> MIVFRYLSREVLVTMSAVSAVLLVIIMSGRFIKYLAQAAQGLLDPGSLFLIMAFRIPGFLQLILPLGLFLGILLAYGRLYLESEMTVLSATGMSQKRLLGYTMAPALLVAILVAWLSLFLAPQGINQFALLLNKQDTLTEFDTLVPGRFQAMRDGTRVTYTEELSKDRGELAGIFISQKDLNSSNQERGISILVAEKGTQNIQADGSRYLILHNGYRYDGNPGQANYRAIQYDTYGVMLPKPEASSEVSERDAVPTADLFGSDNPRYQAELQWRLSTPLLVFVVTLLAVPLSRVNPRQGRFLKLLPAILLYMGYLALLIAVRGQLDKGKIPMAIGLWWVH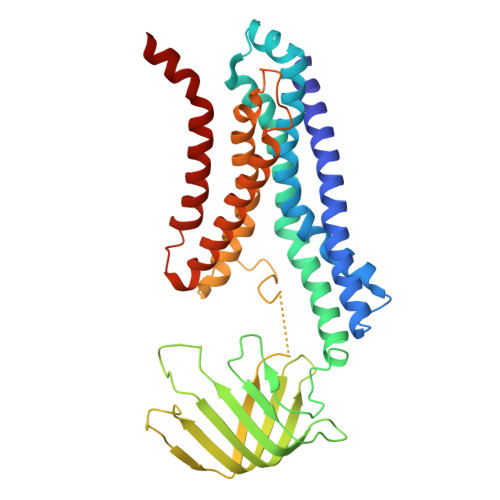GLFLAIGLLLFYWEPLRLKLAS> GPDDPLVINGEIEIVTRAPTPAHLADRFDEIRSGWTFRTDDTQALEMDDFENSGMVFVEEARAVWDRPEGTEGKACADCHGAVDDGMYGLRAVYPKYVESAGKVRTVEQMINACRTSRMGAPEWDYIGPDMTAMVALIASVSRGMPVSVAIDGPAQSTWEKGREIYYTRYGQLDLSCASCHEQYFDHYIRADHLSQGQINGFPSYRLKNARLNAVHDRFRGCIRDTRGVPFAVGSPEFVALELYVASRGNGLSVEGPSVRN;> AEVAPGDVAIDGQGHVARPLTDAPGDPVEGRRLMTDRSVGNCIACHEVTEMADAQFPGTVGPSLDGVAARYPEAMIRGILVNSKNVFPETVMPA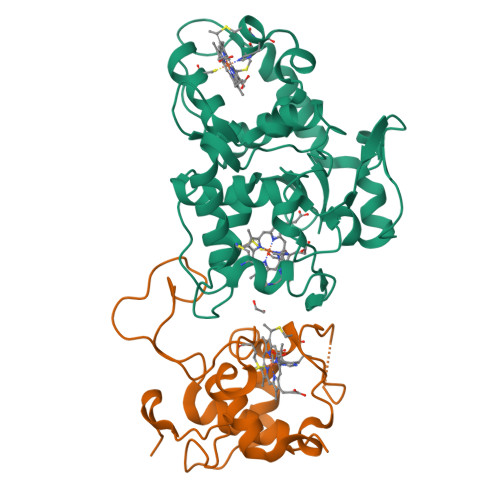YYRVEGFNRPGIAFTSKPIEGEIRPLMTAGQIEDVVAYLMTLTQ> SMSLNIITVTLNMEKYNFLGISIVGQSNERGDGG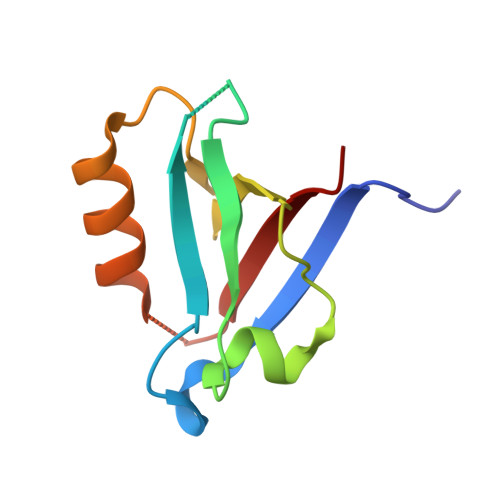IYIGSIMKGGAVAADGRIEPGDMLLQVNDMNFENMSNDDAVRVLRDIVHKPGPIVLTVAKC>MALSTATKAATDALAANRAPTSVNAQEVHRWLQSFNWDFKNNRTKYATKYKMANETKEQFKLIAKEYARMEAVKDERQFGSLQDALTRLNAGVRVHPKWNETMKVVSNFLEVGEYNAIAATGMLWDSAQAAEQKNGYLAQVLDEIRHTHQCAYVNYYFAKNGQDPAGHNDARRTRTIGPLWKGMKRVFSDGFISGDAVECSLNLQLVGEACFTNPLIVAVTEWAAANGDEITPTVFLSIETDELRHMANGYQTVVSIANDPASAKYLNTDLNNAFWTQQKYFTPVLGMLFEYGSKFKVEPWVKTWDRWVYEDWGGIWIGRLGKYGVESPRSLKDAKQDAYWAHHDLYLLAYALWPTGFFRLALPDQEEMEWFEANYPGWYDHYGKIYEEWRARGCEDPSSGFIPLMWFIENNHPIYIDRVSQVPFCPSLAKGASTLRVHEYNGEMHTFSDQWGERMWLAEPERYECQNIFEQYEGRELSEVIAELHGLRSDGKTLIAQPHVRGDKLWTLDDIKRLNCVFKNPVKAFN[2x];>MSMLGERRRGLTDPEMAAVILKALPEAPLDGNNKMGYFVTPRWKRLTEYEALTVYAQPNADWIAGGLDWGDWTQKFHGGRPSWGNETTELRTVDWFKHRDPLRRWHAPYVKDKAEEWRYTDRFLQGYSADGQIRAMNPTWRDEFINRYWGAFLFNEYGLFNAHSQGAREALSDVTRVSLAFWGFDKIDIAQMIQLERGFLAKIVPGFDESTAVPKAEWTNGEVYKSARLAVEGLWQEVFDWNESAFSVHAVYDALFGQFVRREFFQRLAPRFGDNLTPFFINQAQTYFQIAKQGVQDLYYNCLGDDPEFSDYNRTVMRNWTGKWLEPTIAALRDFMGLFAKLPAGTTDKEEITASLYRVVDDWIEDYASRIDFKADRDQIVKAVLAGLK[2x];>MAKLGIHSNDTRDAWVNKIAQLNTLEKAAEMLKQFRMDHTTPFRNSYELDNDYLWIEAKLEEKVAVLKARAFNEVDFRHKTAFGEDAKSVLDGTVAKMNAAKDKWEAEKIHIGFRQAYKPPIMPVNYFLDGERQLGTRLMELRNLNYYDTPLEELR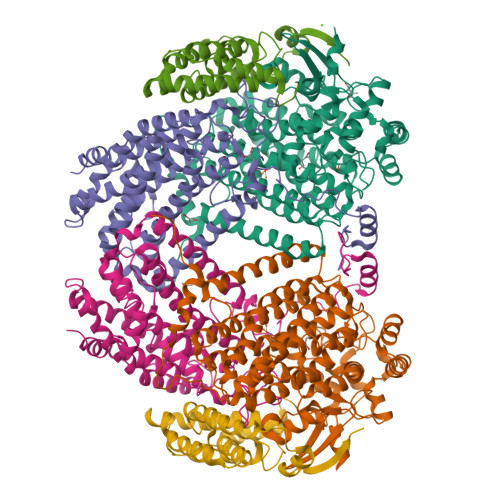KQRGVRVVHLQSPH[2x]>SFKAAGTSGLILKRCSEPERYCLARLMADALRGCVPAFHGVVERDGESYLQLQDL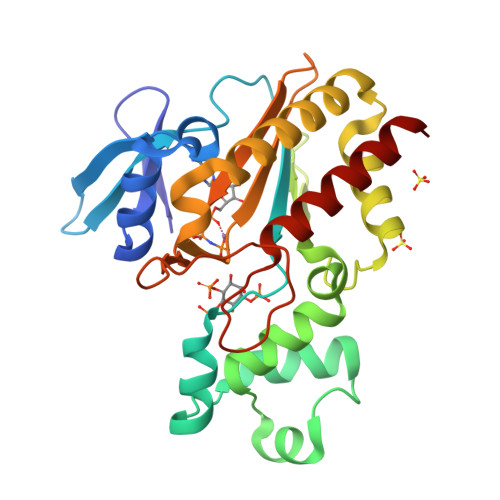LDGFDGPCVLDCKMGVRTYLEEELTKARERPKLRKDMYKKMLAVDPEAPTEEEHAQRAVTKPRYMQWREGISSSTTLGFRIEGIKKADGSCSTDFKTTRSREQVLRVFEEFVQGDEEVLRRYLNRLQQIRDTLEVSEFFRRHEVIGSSLLFVHDHCHRAGVWLIDFGKTTPLPDGQILDHRRPWEEGNREDGYLLGLDNLIGILASLAER[2x]>[6x]MSSRLLPPNRSSLERSLGDVLPAELPVPLRELHDPARCEAALLPYLAWTRSVDRWDPDWSDEAKRNAVATSFVLHQRKGTLTALRQVVEPIGALSEVTEWWQRSPTGVPGTFEITVDVSDRGIDEGTVLELERLLDDVRPVSRHLTRLDLRITPVIRSRHGLAVTDGDTLEIFPWKQ;>[6x]MATTCRTADGDMLDSLCYHVYGHLLGCVEATLDANPGLADEQQPFRAGLLISFPDMPVVNVEQVRLWD;>MSFFHGVTVTNVDIGARTIALPASSVIGLCDVFTPGAQASAKPNVPVLLTSKKDAAAAFGIGSSIYLACEAIYNRAQAVIVAVGVETAETPEAQASAVIGGISAAGERTGLQALLDGKSRFNAQPRLLVAPGHSAQQAVATAMDGLAEKLRAIAILDGPNSTDEAAVAYAKNFGSKRLFMVDPGVQVWDSA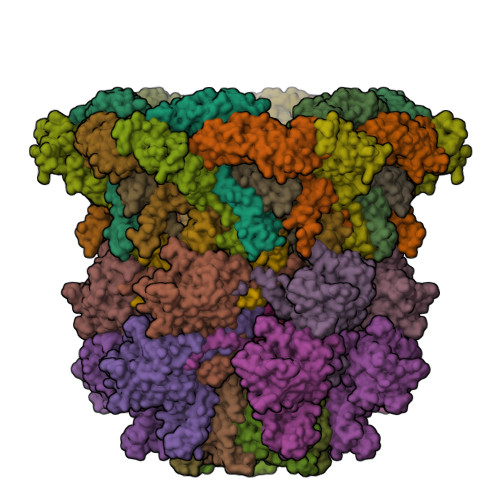TNAARNAPASAYAAGLFAWTDAEYGFWSSPSNKEIKGVTGTSRPVEFLDGDETCRANLLNNANIATIIRDDGYRLWGNRTLSSDSKWAFVTRVRTMDLVMDAILAGHKWAVDRGITKTYVKDVTEGLRAFMRDLKNQGAVINFEVYADPDLNSASQLAQGKVYWNIRFTDVPPAENPNFRVEVTDQWLTEVLDVA[12x];>MIPQTLTNTNLFIDGVSFAGDVPSLTLPKLAVKTEQYRAGGMDAPVSIDMGLEAMEAKFSTNGARREALNFFGLADQSAFNGVFRGSFKGQKGASVPVVATLRGLLKEVDPGDWKAGEKAEFKYAVAVSYYKLEVDGREVYEIDPVNGVRAINGVDQLAGMRNDLGL[12x];>MIGMDRRSGLPLSGLAHLKQSVEDILTTPLGSRRMRPEYGSKLRRMVDMPVSEGWKSAVQAEVARSLGRWEPRIGLSAVRVVAVVDGRVDLLLSGVFEGENINMEVSA[6x];>[6x]MAYLEQLQAGLRYLGRAGESGRKSLDKVVAPVNGAISEIRGAAAELENLPGVSPEMAARLQRAMRGIGQAQGKVNRVVSTYDRASRALLGIDERLDALKVQVNSAAQAVGKVAGDISPTLAGVLPSWLLAPSATPPSEAAASLPHLLVLQPLTANAQPFYFNLNTAAFDALQRNSAYNWSGQVRLGRRPALQSVGMGEESILLKGAVFPLRRQVGNQEKVVGLEQLEALRRLAERREPLILSSGYGEVQMGLWCLVRISENQSALLGNGAPRKQTFDLEFKRYGDDLPNR;>MIIDLSQLPEPEVIENLDFETIYQELLGDFREAMAGEWTAEVESDPVLKLLQLAAYRELLLRARINDAARAVMLAYASGADLDQIGAGFNVQRLLIRPAQPEAVPPVEAQYESDKSLRNRIQLAFEQLSVAGPRNAYIAHALGADGRVADASATSPAPCEVLISVLGVEGNGQAPEAVLQAVRLALNAEDVRPVADRVTVRSAGIVPYQVKAQLYLFPGPEAELIRAAAEASLRDYISAQRRLGRDIRRSALFATLHVEGVQRVELQEPAADVVLDETQAAYCTGYAITLGGVDE[12x]> GSHMAARRGALIVLEGVDGAGKSTQSRKLVEALCAAGHRAELLRFPERSTEIGKLLSSYLQKKSDVEDHSVHLLFSA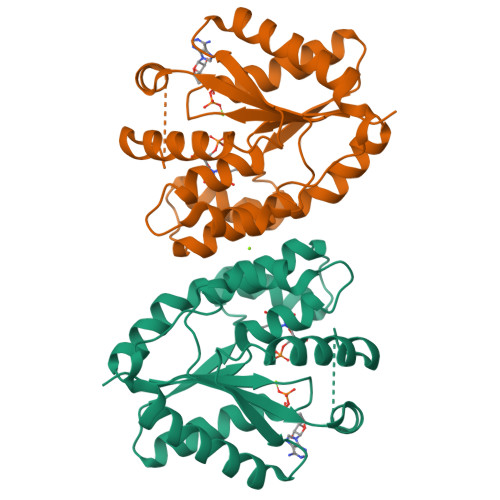NRWEQVPLIKEKLSQGVTLVVDRYAFSGVAFTGAKENFSLDWCKQPDVGLPKPDLVLFLQLQLADAAKRGRARGELERYENGAFQERALRCFHQLMKDTTLNWKMVDASKSIEAVHEDIRVLSEDAIATATEKPLGELWK>AFSWRDAVVYQVYLRSFRDANGDGIGDLGGLSQGLDAIAALGCDAIWLNPCYASPQRDHGYDIADYLTIDPAYGTLEEFDEVVRRAHELGLRVLMDMVANHCSSDHAWFQAALAAEPGSDERARFIFRDGLGPDGELPPNNWDSVFGGLAWTRVTERDGRPGQWYLHSFDTSQPDFDWRHPAVAEHFENVLRFWFERGVDGFRIDVAHGHFKDAALPDHPGGRGPDAGHNHGMWDQPEVHDLYRSWRALGDAYEPEKYFVGEIWVPSPDRLADYLRPDELHNAFSFDLLVQPWNADRFRKAIETGLAVGRGWPAWTLANHDVHRAVTRYGQEQPLDEALPT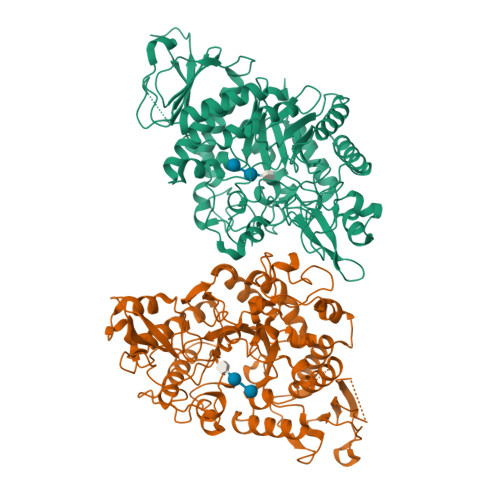DMIAAARRRGPADLDRGLRRARAAAALALALPGSMYLYQGEELGLPEVLDLPDAARQDPIWTRSNGTELGRDGCRIPLPWTREGRTFGFSDAAAATTWLPQPAWFGAFARATQAADPDSMLSLHRDLLATRRTHLRGTEPIVWLSPAGAEVLAFRRGDVVVVTNFGSAPFTPPSAWGALSPLLASQPLTGSATVPPETTVWSRLHRGVA[2x]> DISEPPLHDFYCSRLLDLVFLLDGSSRLSEAEFEVLKAFVVDMMEQLRISQKWVRVAVVEYHDGSHAYIGLKDRKRPSELRRIASQVKYAGSQVASTSEVLKYTLFQIFSKIDRPEASRIALLLMASQEPQRMSRNFVRYVQGLKKKKVIVIPVGIGPHANLKQIRL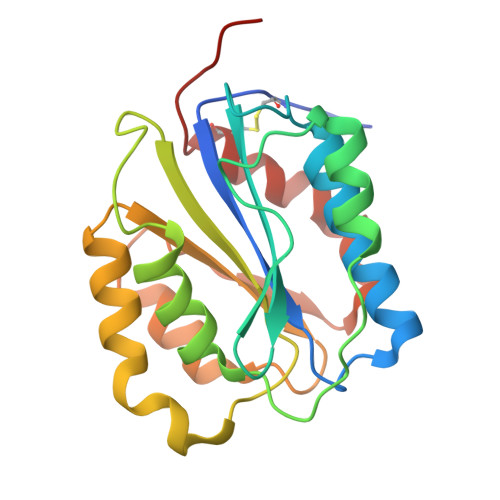IEKQAPENKAFVLSSVDELEQQRDEIVSYLCDLAPEAPPPT> GPIPTAPRENSLMFLSTLPDDTVPAYGNVRTPPVNYLPGEITDLLQLARIPTLMAFERVPEPVPASDTYVPYVAVPTQFDDRPLISFPITLSDPVYQNTLVGAISSNFANYRGCIQITLTFCGPMMARGKFLLSYSPPNGTQPQTLSEAMQCTYSIWDIGLNSSWTFVVPYISPSDYRETRAITNSVY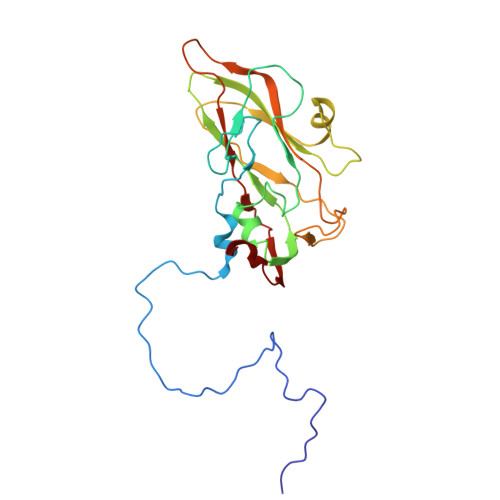SADGWFSLHKLTKITLPPDCPQSPCILFFASAGEDYTLRLPVDCNPSYVF> MFRSSFCKNLENATSHLRLEPDWPSILLICDEINQKDVTPKNAFAAIKKKMNSPNPHSSCYSLLVLESIVKNCGAPVHEEVFTKENCEMFSSFLESTPHENVRQKMLELVQTWAYAFRSSDKYQAIKDTMTILKAKGHTFPELREADAMFTADTAPNWADGRVCHRCRVEFTFTNRKHHCRNCGQVFCGQCTAKQCPLPKYGIEKEVRVC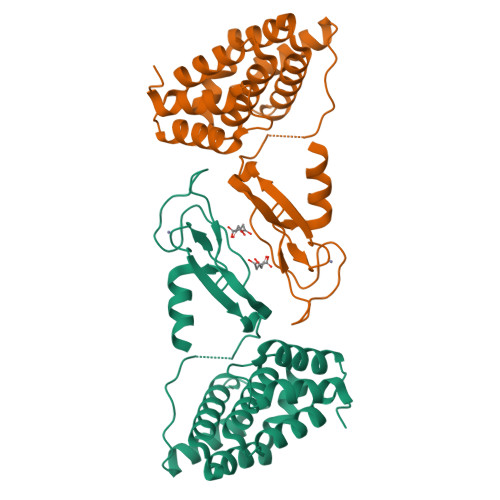DGCFAALQRG>[4x]MAHHHHHHVDDDDKMLLPETRN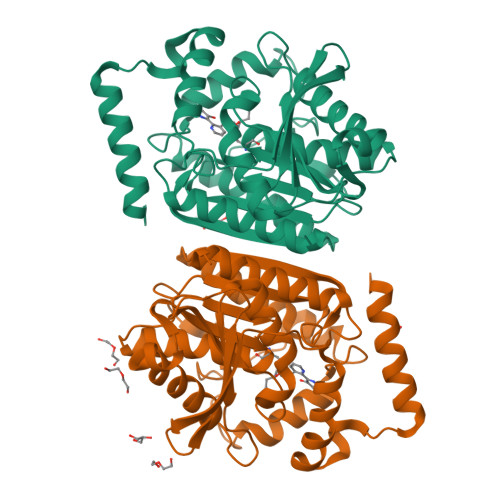LLDLMDAATRGGRPGLDTLPHAVGRKAVDKMSEDGEADPPEVAEVANGGFAGPASEIRFRRYRPLGEAAGLLPTLIYYHGGGFVIGNIETHDSTCRRLANKSRCQVISIDYRLAPEHPFPAPIDDGIAAFRHIRDNAESFGADAARLAVGGDSAGGAMAAVVCQACRDAGETGPAFQMLIYPATDSSRESASRVAFAEGYFLSKAHMDWFWEAYVPEDTDLTDLRLSPLLATDFTGLPPAFVLTAGYDPLRDEGRAYADRLIEAGIKTTYVNYPGTIHGFFSLTRFLSQGLKANDEAAAVMGAHFGT6-methylquinoxaline | C13 H18 N4 | 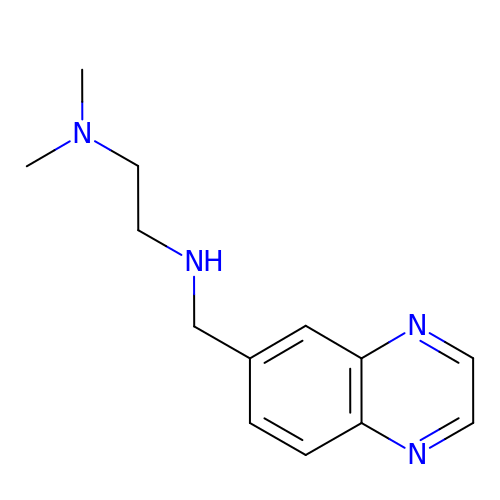OZUJBFNDMZPDCX-UHFFFAOYSA-N> MAEQVALSRTQVCGILREELFQGDAFHQSDTHIFIIMGASGDLAKKKIYPTIWWLFRDGLLPENTFIVGYARSRLTVADIRKQSEPFFKATPEEKLKLEDFFARNSYVAGQYDDAASYQRLNSHMNALHLGSQANRLFYLALPPTVYEAVTKNIHESCMSQIGWNRIIVEKPFGRDLQSSDRLSNHISSLFREDQIYRIDHYLGKEMVQNLMVLRFANRIFGPIWNRDNIACVILTFKEPFGTEGRGGYFDEFGIIRDVMQNHLLQMLCLVAMEKPASTNSDDVRDEKVKVLKCISEVQANNVVLGQYVGNPDGEGEATKGYLDDPTVPRGSTTATFAAVVLYVENERWDGVPFILRCGKALNERKAEVRLQFHDVAGDIFHQ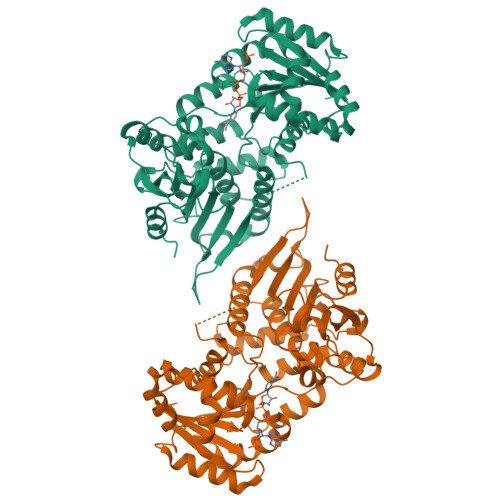QCKRNELVIRLQPNEAVYTKMMTKKPGMFFNPEESELDLTYGNRYKNVKLPDAYERLILDVFCGSQMHFVRSDELREAWRIFTPLLHQIELEKPKPIPYIYGSRGPTEADELMKRVGFQYEGTYKWVNPHKL>MTADGPRELLQLRAAVRHRPQDFVAWLMLADAELGMGDTTAGEMAVQRGLALHPGHPEAVARLGRVRWTQQRHAEAAVLLQQASDAAPEHPGIALWLGHALEDAGQAEAAAAAYTRAHQLLPEEPYITAQLLNWRRRLCDWRALDVLSAQVRAAVAQGVGAVEPFAFLSEDASAAEQLACARTRAQAIAASVRPLAPTRVRSKGPLRVGFVSNGFGAHPTGLLTVALFEALQRRQPDLQMHLFATSGDDGSTLRTRLAQASTLHDVTALGHLATAKHIRHHGIDLLFDLAGWGGGGRPEVFALRPAPVQVNWLAYPGTSGAPWMDYVLGDAFALPPALEPFYSEHVLRLQGAFQPSDTSRVVAEPPSRTQCGLPEQGVVLCCFNNSYKLNPQSMARMLAVLREVPDSVLWLLSGPGEADARLRAFAHAQGVDAQRLVFMPKLPHPQYLARYRHADLFLDTHPYNAHTTASDALWTGCPVLTTPGETFAARVAGSLNHHLGLDEMNVADDAAFVAKAVALASDPAALTALHARVDVLRRASGVFHMDGFADDFG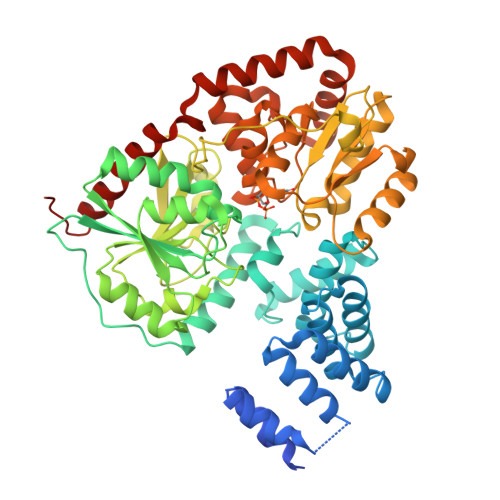ALLQALARRHGWLGI[2x]> MGHHHHHHGGMLRFVRGNL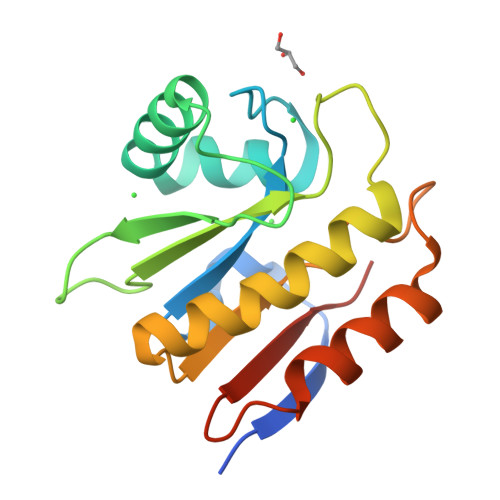LEAPVEALVNTVNTVGVMGKGVALQFKRAFPDNYQAYVKACERGQVQIGRIFVYDRGPLAQPRYIFNFPTKKHWRHPSRMEYVEEGLKDLVCRIQELRVRSIALPPLGAGNGGLPWPEVKQRIQEALEALEGVEVWVYEPVENPKA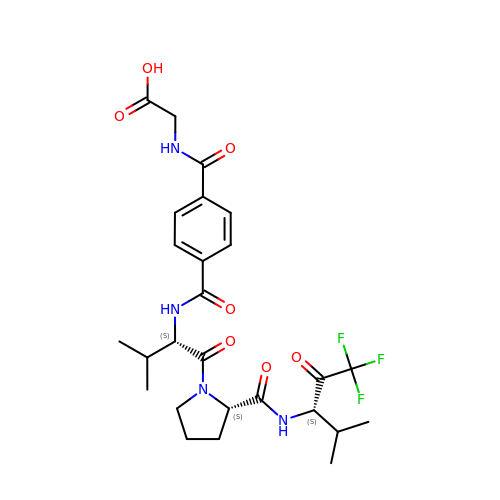2-[4-[[(S)-1-[[(S)-2-[[(RS)-3,3,3-TRIFLUORO-1-ISOPROPYL-2-OXOPROPYL]AMINOCARBONYL]PYRROLIDIN-1-YL-]CARBONYL]-2-METHYLPROPYL]AMINOCARBONYL]BENZOYLAMINO]ACETIC ACID | C26 H33 F3 N4 O7 | MRTSIBBMOWLRPY-IHPCNDPISA-N Coxsackievirus A10 (CV-A10) belongs to the enterovirus genus in the Picornaviridae family. The virus is considered one of the major causative agents of hand, foot, and mouth disease (HFMD), which is highly infectious and affects millions of young children annually. In general, enteroviral capsids are composed of 60 copies of biological protomers that are arranged in a pseudo-T = 3 icosahedral symmetry. Each protomer consists of four capsid proteins, including VP1, VP2, VP3, and VP4.

In the present study, we determined the structures of CV-A10 mature virion and NEP at 2.84 and 3.12 Å, respectively, by cryo-EM single-particle analysis. The cryo-EM map of mature virion displays surface features typical for enteroviruses, including a “mesa” at five-fold symmetry axis, a “canyon” around the mesa, and a three blade “propeller” at three-fold symmetry axis. In the mature virion, most of the surface exposed hydrophilic loops, including the BC, EF, and GH loops of VP1 and the EF loop of VP2 are well resolved, whereas the densities for a few residues (including residues 1, 10–17, and 297 of VP1, residues 1–10 of VP2, and residues 1–27 and 69 of VP4) are missing. Similar to other enteroviruses, CV-A10 virion also displays the canyon feature surrounding the five-fold axis, which appears to be shallower and narrower than that in EV-A71, CV-A16, and poliovirus type 1 (PV-1). Specifically, the VP1 BC loop shows obviously distinct conformations in CV-A10 compared with those in EV-A71 and CV-A16, and the VP1 GH loop of CV-A10 does not have the typical small α-helix as in EV-A71 and CV-A16, but forms a loop, probably due to the presence of Pro213 in the VP1 GH loop of CV-A10, which may have disrupted the α-helix formation. In our CV-A10 mature virion map, density corresponding to a pocket factor can be clearly observed inside the “pocket”. According to our mature virion cryo-EM structure, the pocket factor of CV-A10 is mostly buried in the hydrophobic pocket of VP1, and its main body forms abundant hydrophobic interactions with surrounding residues, whereas its head forms hydrogen bonds with residues near the entrance and middle position of the pocket, including Ile109, Ile111, and Asn226. Our CV-A10 mature virion structure revealed the presence of a pocket factor corresponding to a fatty acid with 18 carbon atoms within the VP1 hydrophobic pocket. The major densities bridging the capsid shell and the RNA shell underneath the three-fold symmetrical axis region and pentamer were identified, and the possible residues involved in capsid interaction with RNA could be Arg43 and Arg62 of VP4, Arg18 of VP1, and to a less extent, Ser10 of VP2. In consistence with this observation, in silico docking showed that the VP1 pocket in CV-A10 could not accommodate WIN51711, pleconaril, or pirodavir due to steric hindrance imposed by some VP1 residues including Phe133, Met193, and Asn226.

> GDPVEDIIHDALGNTARRAISGATNVESAADTTPSSHRLETGRVPALQAAETGATSNATDENMIETRCVINRNGVLETTINHFFSRSGLVGVVNLTDGGDTTGYATWDIDIMGFVQLRRKCEMFTYMRFNAEFTFVTTTKSGEARPYMLQYMYVPPGAPKPTGRDAFQWQTATNPSVFVKLTDPPAQVSVPFMSPASAYQWFYDGYPTFGQHPETSNTTYGLCPNNMMGTFAVRVVSREASQLKLQTRVYMKLKHVRAWVPRPIRSQPYLLKNFPNYDSSKITNSARDRSSIKQANM;> SPSVEACGYSDRVAQLTVGNSSITTQEAANIVLAYGEWPEYCPDTDATAVDKPTRPDVSVNRFYTLDSKMWQENSTGWYWKFPDVLNKTGVFGQNAQFHYLYRSGFCLHVQCNASKFHQGALLVAVIPEFVIAGRGSNTKPNEAPHPGFTTTFPGTTGATFHDPYVLDSGVPLSQALIYPHQWVNLRTNNCATVIVPYINAVPFDSAINHSNFGLVVVPVSPLKYSSGATTAIPITITIAPLNSEFGGLRQAVSQ;> GIPAELRPGTNQFLTTDDDTAAPILPGFTPTPTIHIPGEVHSLLELCRVETILEVNNTTEATGLTRLLIPVSSQNKADELCAAFMVDPGRIGPWQSTLVGQICRYYTQWSGSLKVTFMFTGSFMATGKMLVAYSPPGSAQPANRETAMLGTHVIWDFGLQSSVSLVIPWISNTHFRTAKTGGNYDYYTAGVVTLWYQTNYVVPPETPGEAYIIAMGAAQDNFTLKICKDTDEVTQQAVLQ;> MGAQVSTQKSGSHETGNVATGGSTINFTNINYYKDSYAASATRQDFTQDPKKFTQPVLDSIRELSAPLN> MGSDKIHHHHHHENLYFQGTHGPALPGVCIFSSPRA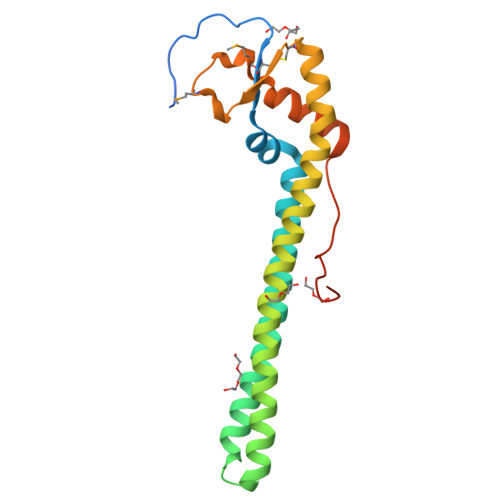VGSSLVGKAVDARLKTIIQQVNAELTGERTALDNEAKALDAKKTTIAQDALEQQAATLQAKANAWQRKGQLRQKEVEATEQKALSRVYQELNTPIQQVYQAQKCSVLLDREAVMLANPAMDITDAVVAALDARIKTLTFDRERLDQQVPGAAALQPTNK>[7x]MQQGQMAYDRAITVFSPDGRLFQVEYAREAVKKGSTALGMKFANGVLLISDKKVRSRLIEQNSIEKIQLIDDYVAAVTSGLVADARVLVDFARISAQQEKVTYGSLVNIENLVKRVADQMQQYTQYGGVRPYGVSLIFAGIDQIGPRLFDCDPAGTINEYKATAIGSGKDAVVSFLEREYKENLPEKEAVTLGIKALKSSLEEGEELKAPEIASITVGNKYRIYDQEEVKKFL;>MNQTLETGTTTVGITLKDAVIMATERRVTMENFIMHKNGKKLFQIDTYTGMTIAGLVGDAQVLVRYMKAELELYRLQRRVNMPIEAVATLLSNMLNQVKYMPYMVQLLVGGIDTAPHVFSIDAAGGSVEDIYASTGSGSPFVYGVLESQYSEKMTVDEGVDLVIRAISAAKQRDSASGGMIDVAVITRKDGYVQLPTDQIESRIRKLGLILHHHHHH[7x];>MHH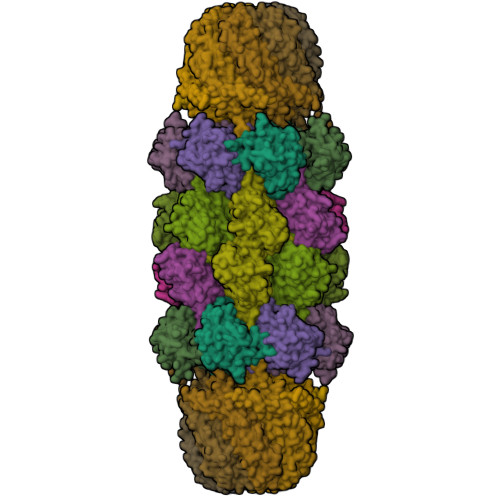HHHHPPKRAALIQNLRDSYTETSSFAVIEEWAAGTLQEIEGIAKAAAEAHGVIRNSTYGRAQAEKSPEQLLGVLQRYQDLCHNVYCQAETIRTVIAIRIPEHKEEDNLGVAVQHAVLKIIDELEIKTLGSGEKSGSGGAPTPIGMYALREYLSARSTVEDKLLGSVDAESGKTKGGSQSPSLLLELRQIDADFMLKVELATTHLSTMVRAVINAYLLNWKKLIQPRTGSDHMVS[7x]> QSIDSGISSLSYNRNEVLASNGDKIESFVPKEGKKAGNKFIVVERQKRSLTTSPVDISI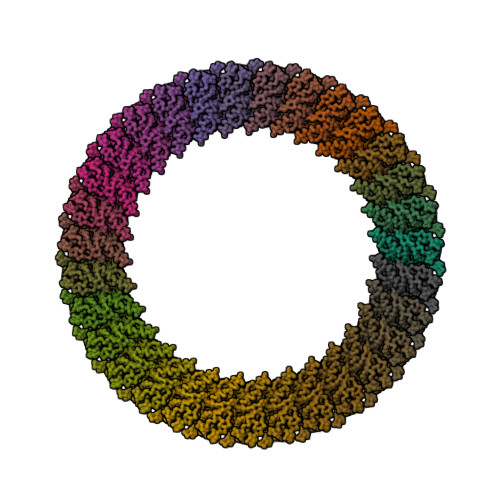IDSVNDRTYPGALQLADKAFVENRPTILMVKRKPININISIKVDDPTYGKVSGAIDELVSKWNEKYSSTHTLPARTQYSESMVYSKSQISSALNVNAKVLENSLGVDFNAVANNEKKVMILAYKQIFYTVSADLPKNPSDLFDDSVTFNDLKQKGVSNEAPPLMVSNVAYGRTIYVKLETTSSSKDVQAAFKALIKNTDIKNSQQYKDIYENSSFTAVVLGGDAQEHNKVVTKDFDEIRKVIKDNATFSTKNPAYPISYTSVFLKDNSVAAVHNKTDYIETTSTEYSKGKINLDHSGAYVAQFEVAWDEVSYDKEGNEVLTHKTWDGNYQDKTAHYSTVIPLEANARNIRIKARECTGLAWEWWRDVISEYDVPLTNNINVSIWGTTLYPGSSITYN> CGFGGSGSNGEGKKDSKGKTTLNINIKTEPFSLHPGLANDSVSGGVIRQTFEGLTRINADGEPEEGMASKIETSKDGKTYTFTIRDGVKWSNGDPVTAQDFEYAWKWALDPNNESQYAYQLYYIKGAEAANTGKGSLDDVAVKAVNDKTLKVELNNPTPYFTELTAFYTYMPINKKIAEKNKKWNTNAGDDYVSNGPFKMTAWKHSGSITLEKNDQYWDKDKVKLKKIDMVMINNNNTELKKFQAGELDWAGMPLGQLP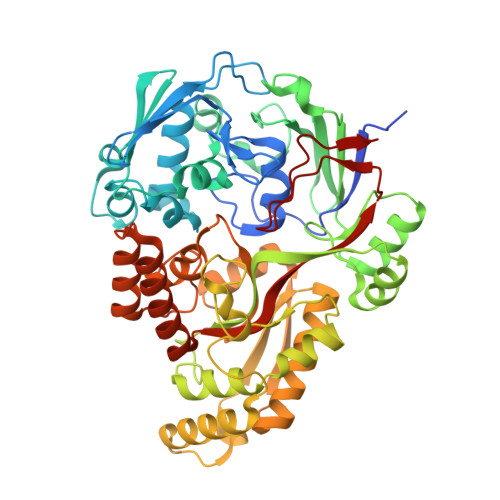TESLPTLKKDGSLHVEPIAGVYWYKFNTEAKPLDNVNIRKALTYSLDRQSIVKNVTQGEQIPAMAAVPPTMKGFEDNKEGYFKDNDVKTAKEYLEKGLKEMGLSKASDLPKIKLSYNTDDAHAKIAQAVQEMWKKNLGVDVELDNSEWNVYIDKLHSQDYQIGRMGWLGDFNDPINFLELFRDKNGGNNDTGWENPEFKKLLNQSQTETDKTKRAELLKKAEGIFIDEMPVAPIYFYTDTWVQDENLKGVIMPGTGEVYFRNAYFK>MSSASGL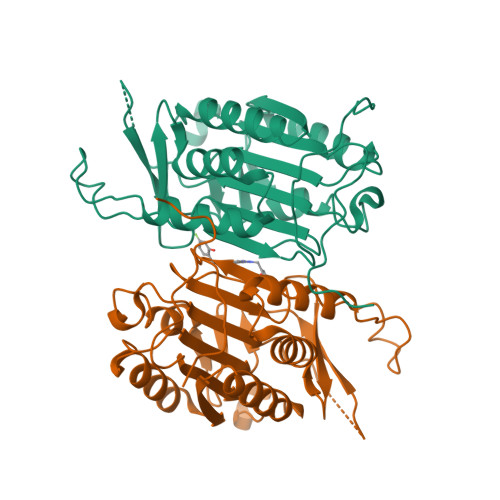RRGHPAGGEENMTETDAFYKREMFDPAEKYKMDHRRRGIALIFNHERFFWHLTLPERRGTCADRDNLTRRFSDLGFEVKCFNDLKAEELLLKIHEVSTVSHADADCFVCVFLSHGEGNHIYAYDAKIEIQTLTGLFKGDKCHSLVGKPKIFIIQAARGNQHDVPVIPLDVVDNQTEKLDTNITEVDAASVYTLPAGADFLMCYSVAEGYYSHRETVNGSWYIQDLCEMLGKYGSSLEFTELLTLVNRKVSQRRVDFCKDPSAIGKKQVPCFASMLTKKLHFFPKSNENLYFQ[4x]N-[2-benzyl-4-(1H-tetrazol-5-yl)phenyl]-6-(cyclohexylmethyl)pyridine-2-carboxamide 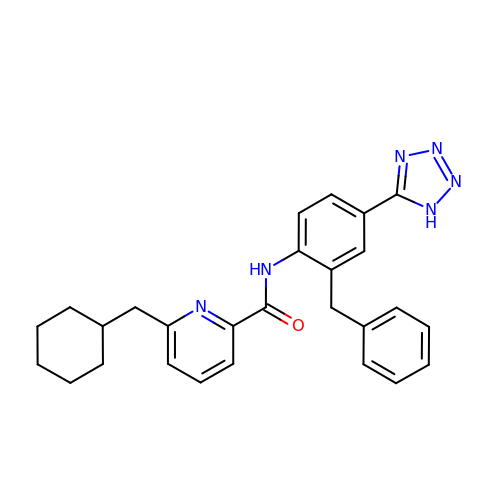| C27 H28 N6 O | DXIJKKFLXBIMCT-UHFFFAOYSA-N>[2x]MSKPIEIEIRRAPVLGSSMAYRETGAQDAPVVLFLHGNPTSSHIWRNILPLVSPVAHCIAPDL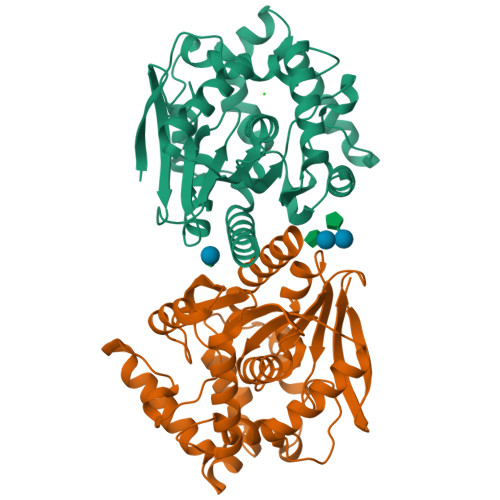IGFGQSGKPDIAYRFFDHVRYLDAFIEQRGVTSAYLVAQDWGTALAFHLAARRPDFVRGLAFMEFIRPMPTWQDFHHTEVAEEQDHAEAARAVFRKFRTPGEGEAMILEANAFVERVLPGGIVRKLGDEEMAPYRTPFPTPESRRPVLAFPRELPIAGEPADVYEALQSAHAALAASSYPKLLFTGEPGALVSPEFAERFAASLTRCALIRLGAGLHYLQEDHADAIGRSVAGWIAGIEAVRPQLAAVD>[2x]SKPFSVPVLTVEEMTNSRFPIPLEKLFTGPSSAFVVQPQNGRCTTDGVLLGTTQLSPVNICTFRGDVTHITGSRNYTMNLASQNWNDYDPTEEIPAPLGTPDFVGKIQGV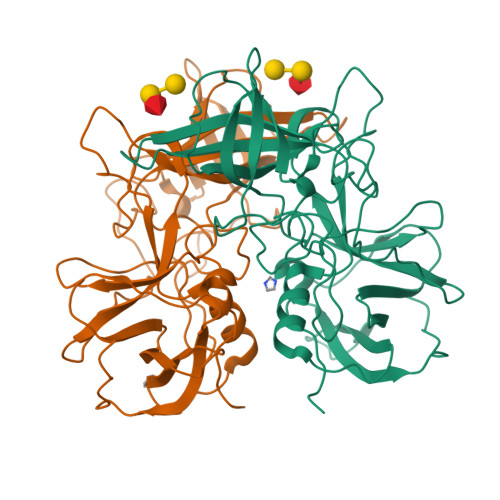LTQTTRTDGSTRGHKATVYTGSADFAPKLGRVQFETDTDRDFEANQNTKFTPVGVIQDGGTTHRNEPQQWVLPSYSGRNTHNVHLAPAVAPTFPGEQLLFFRSTMPGCSGYPNMDLDCLLPQEWVQYFYQEAAPAQSDVALLRFVNPDTGRVLFECKLHKSGYVTVAHTGQHDLVIPPNGYFRFDSWVNQFYTLAPM> VPPALHLVDPQIQLTITADPKVYPIILRLGSNLSLSMARRNLDSLEARAFQSTPIVVQMTKLATTEELPDEFVVVTAK;> VPPALHLVDPQIQLTITRADPKVYPIILRLGSNLSLSMARRNLDSLEARAFQSTPIVVQMTKLATTEELPDEFVVVTAK;>PPALHLVDPQIQLTITDPKVYPIILRLGSNLSLSMARRNLDSLEARAFQSTPIVVQMTKLATTEELPD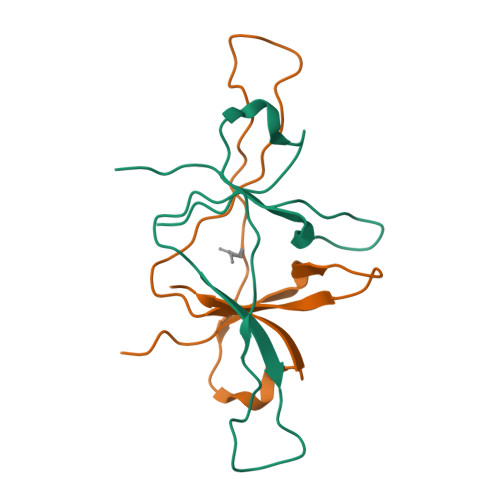EFVVVTAK[4x];>[2x]VPPALHLVDPQIQLTITDPKVYPIILRLGSNLSLSMARRNLDSLEARAFQSTPIVVQMTKLATTEELPDEFVVVTAK> MSRVFRVPLAPTRGGATTAPRTPAPAPAPTRPGIVAGCLSPHPPHLIYGENPPQNEPRSTGGWETLRWAYERLRARIRDVHKPDVLIVHAPHWITMVGHHVNCVPNPRGLSVEPIFPHLFRYRYDFRTDVELGEAIAEEASGLGLVTRTLRDPRVRVDYATIGALHLANPAWDIPVVSLSANNNP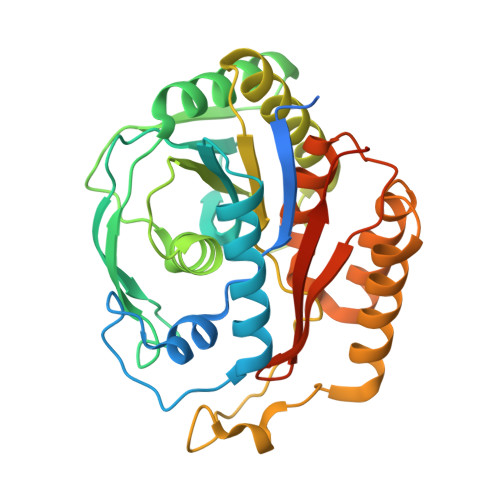YFYSDASLTEMEVLGEATRLAVEATGRRAVLLASNSLSHLHWHEEPELPEDMEREHPYNNHQYRWDMKLLEAIRRGPTAPLRDLIPEHIEATASETKAGSLTWMLAAMGWPKVAGDVLGYGTIIGTGNAIVEWLPEGSHHGGSGGSHHHHHH>MSSINKPLRLIFPQWQGGDNPPYYLGSQLLAWLSPDPKGAVEEVPVPKPTGEPLQEENGIVGRSILIDQLSEARQLIEKHTPDSLVVLGGDCLVSLAPFSWLLEKYKDKLGILWIDSHPDVQTPKEYKNAHAHVLGELMGNGDSDFTRTVKHPVSPQKIMIAGIHDPLPYEANFISEHKIQTCSPEQVRSGAQPVLDWIKNEKIEYLAIHIDLDVLDPHNFRSVLFAKPGRGQHDFGDVAEGKLNIPDVVKLANQAASISKAVGLTIAEHLPWDALNLKNMLEELPL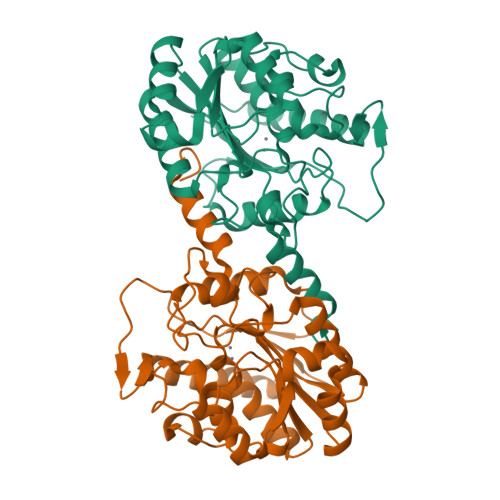IGK[4x]> MAGNMLANYVQVYVMLPLDVVSVDNKFEKGDEIRAQLKKLTEAGVDGVMIDVWWGLVEGKGPKAYDWSAYKQVFDLVHEAGLKLQAIMSFHQCGGNVGDVVNIPIPQWVRDVGATDPDIFYTNRGGTRNIEYLTLGVDDQPLFHGRTAVQMYADYMASFRENMKKFLDAGTIVDIEVGLGPAGEMRYPSYPQSQGWVFPGIGEFICYDKYLEADFKAAAAKAGHPEWELPDDAGEYNDTPEKTQFFKDNGTYLTEKGKFFLSWYSNKLIKHGDKILDEANKVFLGCRVQLAIKISGIHWWYRVPNHAAELTAGYYNLDDRDGYRTIARMLTRHHASMNFTCAEMRDSEQSEEAKSAPEELVQQVLSAGWREGLHVACENALGRYDATAYNTILRNARPKGINKNGPPEHKLFGFTYLRLSNELLEGQNYATFQTFVEKMHANLGHDPSVDPVAPLERSKPEMPIEMILKAAQPKLEPFPFDKNTDLPVKDHTDVGDEVLVAPVHHHHHH

The wheat β‐amylase (Tri a 17) has been found to bind IgE of wheat allergic patients, but its structure and allergenic activity have not been studied. To evaluate its possible clinical relevance and to shed some light on its biochemical properties, we elucidated the three‐dimensional structure, measured the enzymatic activity, IgE‐binding capacity, and allergenic activity of the recombinant enzyme. The β‐amylases of crop plants like wheat, soy, or barley have been under investigation for decades and the presence of two general forms has been described. One protein isoform found in all parts of the plant, termed ubiquitous β‐amylase, and one variant specific to the endosperm, featuring an elongated C‐terminal tail region are known.

A refolding attempt yielded soluble, yet misfolded and aggregated protein. However, we were able to optimize the expression conditions to obtain natively folded amylase (named Tri a 17_active) (Figure S1 and S2 and the Methods section in this article's Online Repository). The far‐UV CD spectra of the inactive proteins indicate the presence of β‐sheets and random coil signal, while Tri a 17_active exhibits the high α‐helical content of a TIM‐barrel. The crystal structure of Tri a 17_active shows the same (β/α)8‐barrel architecture found for other plant and bacterial β‐amylases. The structure superimposes well with the previously published structure of barley β‐amylase (rmsd = 0.62 Å when 442 of 486 Cα atoms are aligned with the PDB structure 2XFF5), which was used as the template for molecular replacement. The enzyme shows a tolerance for low pH, showing maximum activity at pH 5 and retaining over 80% of its maximum activity even at pH 4. In general, Tri a 17 is highly active in a wide range of acidic pH conditions (4.0‐7.0), similar to other β‐amylases, such as the major β‐amylases of barley. The protein is most stable in slightly acidic conditions. A maximum in melting temperature is seen at pH 5.5 with 59°C, with a tail off to lower values as pH increases and a sharp drop in stability at pH 4. Tri a 17_clone and Tri a 17_inactive were recognized by 24% (4 of 17) of wheat food allergic patients with varying intensities, whereas the folded enzyme (Tri a 17_active) was recognized by 41% (7 of 17) of wheat food allergic patients, indicating the presence of conformational IgE epitopes as well as linear epitopes. Since the enzymatic activity depends on the correct fold, there is an apparent correlation between enzymatic and allergenic activity of the β‐amylase.> MHHHHHHHAVRASEISRVYEAYPEKKATLYFLVLGFLALIVGSLFGPFQALNYGNVDAYPLLKRLLPFVQSYYQGLTLHGVLNAIVFTQLFAQAIMVYLPARELNMRPNMGLMWLSWWMAFIGLVVFALPLLANEATVLYTFYPPLKGHWAFYLGASVFVLSTWVSIYIVLDLWRRWKAANPGKVTPLVTYMAVVFWLMWFLASLGLVLEAVLFLLPWSFGLVEGVDPLVARTLFWWTGHPIMYFWLLPAYAIIYTILPKQAGGKLVSDPMARLAFLLFLLLSTPVGFHHQFADPGIDPTWKMIHSVLTL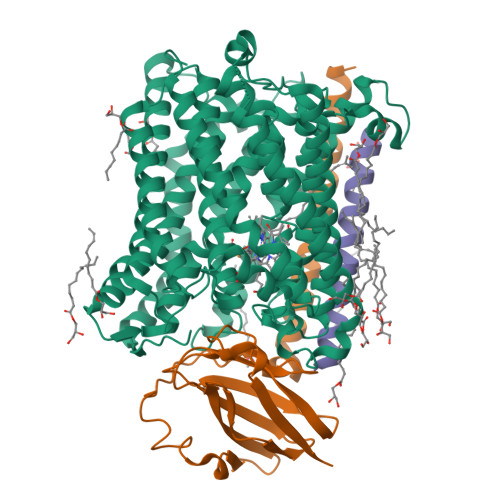FVAVPSLMTAFTVAASLEFAGRLRGGRGLFGWIRALPWDNPAFVAPVLGLLGFIPGGAGGIVNASFTLDYVVHNTAWVPGHFHLQVASLVTLTAMGSLYWLLPNLTGKPISDAQRRLGLAVVWLWFLGMMIMAVGLHWAGLLNVPRRAYIAQVPDAYPHAAVPMVFNVLAGIVLLVALLLFIYGLFSVLLSRERKPELAEAPLPFAEVISGPEDRRLVLAMDRIGFWFAVAAILVVLAYGPTLVQLFGHLNPVPGWRLW;> MVDEHKAHKAILAYEKGWLAFSLAMLFVFIALIAYTLATHTAGVIPAGKLERVDPTTVRQEGPWADPAQAVVQTGPNQYTVYVLAFAFGYQPNPIEVPQGAEIVFKITSPDVIHGFHVEGTNINVEVLPGEVSTVRYTFKRPGEYRIICNQYCGLGHQNMFGTIVVKE;> MEEKPKGALAVILVLTLTILVFWLGVYAVFFARG>[12x]MMENINIVIKDVGYFQDKPQFLNSKSVRQWKHGTKVKLTKHNSHWYTGVVKDGNKSVRGYIYHSMAKVTSKNSDGSVNATINAHAFCWDNKKL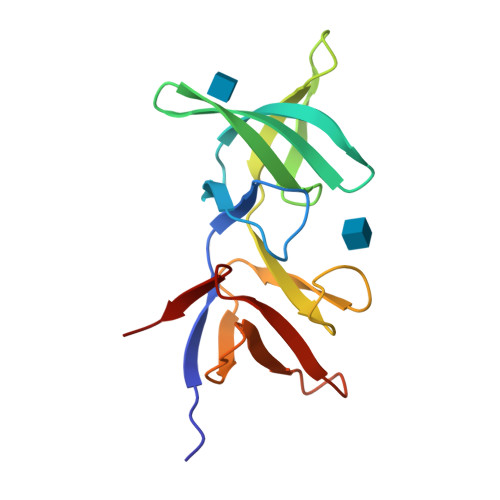NGGDFINLKRGFKGITHPASDGFYPLYFASRKKTFYIPRYMFDIKK Pyruvate carboxylase (PC) is a tetrameric enzyme that contains two active sites per subunit that catalyze two consecutive reactions. A mobile domain with an attached prosthetic biotin links both reactions, an initial biotin carboxylation and the subsequent carboxyl transfer to pyruvate substrate to produce oxaloacetate. PC is mostly found as tetramers of four identical subunits, with monomers of ~120–130 kDa in size. This enzyme possesses a tetrahedral geometry with the tetramer organized in two layers. In this work, we study the structure of Lactococcus lactis PC (LlPC) during catalysis in the presence of positive allosteric regulator acetyl-CoA.

We obtained a cryo-EM map of LlPC with acetyl-CoA under reaction conditions with an estimated global resolution of 2.12 Å. This resolution should allow the identification of side chains, the substrates and products of the reactions, and even ions and water molecules. However, there are large differences in resolution throughout the protein as observed in local resolution estimates. This initial map is a mixture of the different conformations of the enzyme during catalysis, and hence, BCCP domains are not visible at the current density threshold. After symmetry expansion of our dataset, the first step of our analysis is the separation of catalytic states at both BC and CT reaction sites of all the subunits. In all the cryoEM maps for LlPC analyzed in this work, the subunits have a symmetrical organization without major differences in their overall architecture. LlPC has a specific activity of 127 min−1 which is slightly increased in the presence of the allosteric regulator acetyl-CoA to 154 min−1. The binding of the allosteric activator acetyl-CoA to this domain modifies the angle between BC and CT domains in 1.4° while the angle between CTs remains unaltered. In summary, we have resolved several catalytic states of LlPC with the allosteric activator acetyl-CoA and the motions that LlPC tetramers undergo during catalysis.

>VPRGSHMKKLLVANRGEIAVRVFRACNELGLSTVAVYAREDEYSVHRFKADESYLIGQGKKPIDAYLDIDDIIRVALESGADAIHPGYGLLSENLEFATKVRAAGLVFVGPELHHLDIFGDKIKAKAAADEAKVPGIPGTNGAVDIDGALEFAKTYGYPVMIKAALGGGGRGMRVARNDAEMHDGYARAKSEAIGAFGSGEIYVEKYIENPKHIEVQILGDRHGNIIHLHERDCSVQRRNQKVIEIAPAVGLSPDFRNEICEAAVKLCKNVGYVNAGTVEFLVKDDKFYFIEVNPRVQVEHTITELITGVDIVQAQILIAQGKDLHREIGLPAQSEIPLLGSAIQCRITTEDPQNGFLPDTGKIDTYRSPGGFGIRLDVGNAYAGYEVTPYFDSLLVKVCTFANEFSDSVRKMDRVLHEFRIRGVKTNIPFLINVIANENFTSGQATTTFIDNTPSLFNFPRLRDRGTKTLHYLSMITVNGFPGIENTEKRHFEEPRQPLLNLEKKKTAKNILDEQGADAVVDYVKNTKEVLLTDTTLRDAHQSLLATRLRLQDMKGIAQAIDQGLPELFSAEMWGGATFDVAYRFLNESPWYRLRKLRKLMPNTMFQMLFRGSNAVGYQNYPDNVIEEFIRVAAHEGIDVFRIFDSLNWLPQMEKSIQAVRDNGKIAEATICYTGDILDPSRPKYNIQYYKDLAKELEATGAHILAVKDMAGLLKPQAAYRLISELKDTVDLPIHLHTHDTSGNGIITYSGATQAGVDIIDVATASLAGGTSQPSMQSIYYALEHGPRHASINVKNAEQIDHYWEDVRKYYAPFEAGITSPQTEVYMHEMPGGQYTNLKSQAAAVGLGHRFDEIKQMYRKVNMMFGDIIKVTPSSKVVGDMALFMIQNDLTEEDVYARGNELNFPESVVSFFRGDLGQPVGGFPEKLQKIIVKDKAVITDRPGLHAEKVDFETVKADLEQKIGYEPGDHEVISYIMYPQVFLDYQKMQREFGAVTLLDTPTFLHGMRLNEKIEVQIEKGKTLSIRLDEIGEPDLAGNRVLFFNLNGQRREVVINDQSVQAQVVAKRKAETGNPNQIGATMPGSVLEILVKAGDKVQKGQALMVTEAMKMETTIEAPFDGEIVDLHVVKGEAIQTQDLLIEIN[4x]> VIVYGDYNND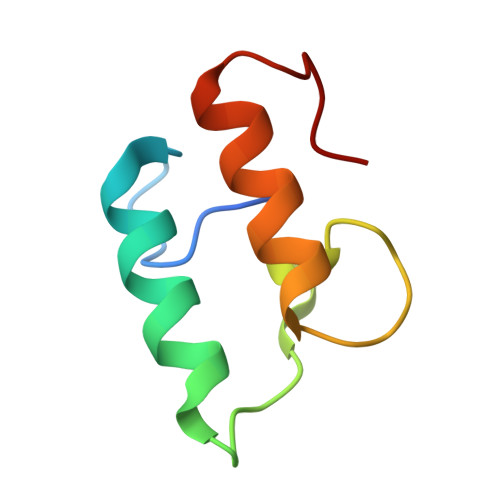GNVDSTDFAGLKKYIMAADHAYVKNLDVNLDNEVNAFDLAILKKYLLGMVSKLE>[4x]UGAGCXCGGCUC

Herein we extend these studies and present a crystal structure that provides detailed conformational information on how the amide is accommodated in the RNA duplex and further illustrates the excellent hydration and conformational adaptability of amide linkages in RNA. Our crystallographic and RNAi activity studies are consistent with earlier biophysical and NMR results and, taken together, strongly suggest that amides are excellent structural mimics of the phosphate backbone in RNA and may have the potential to improve the properties of siRNAs. The present crystal structure provides unique insights into the conformation and hydration of the amide linkage and confirms our earlier observations that AM1 amide is surprisingly efficient in mimicking the phosphate backbone in RNA. The amide linkages are not only tolerated at internal positions of both guide and passenger strands of siRNAs, but may also increase the silencing activity when placed near the 5′-end of the passenger strand.

Out of several self-complementary RNAs with a single isolated amide linkage we synthesized for crystallography studies, RNA 13mer rUGAGCUAM1UCGGCUC (abbreviated RNA13) gave well diffracting crystals. The circular dichroism spectra had significant differences but were not expected to be similar because of different conformations of the respective crystal structures. This 13mer features non-canonical UoG wobble and U*C base pairs in the middle of the duplex and 5′-terminal U overhangs. The space group was P1 with two 13mer duplexes in the unit cell. Two partially occupied strontium ions were retrieved and the experimental density allowed building of complete models of the two duplexes without the dangling Us. Their structures along with 269 water molecules were refined to an R-factor of 17.1% (R-free 23.5%) at a resolution of 1.2 Å. The RNA13 duplex adopts an A-like conformation with modulated groove widths as a result of the UoG wobble and U*C pairs in the central part. The conformation of RNA13 differs significantly from that displayed by the native RNA 13mer. Amide moieties in all four strands assume similar conformations. The structure reveals that the amide carbonyl group is rotated into the major groove and thus assumes an orientation that is similar to that of the P–OP2 bond. Compared with the distances between adjacent OP2 atoms (as short as 5 Å), the distances between amide carbonyl oxygen and OP2s from 5′- and 3′-adjacent residues are slightly longer (ca. 6 Å), resulting in tandem waters linking the carbonyl group and phosphate oxygens.> XADVAGTSNRDFRGREQRLFNSEQYNYNNSLNGEVSVWVYAYYSDGSVLVINKNSQYKVGISETFKALKEYREGQHNDSYDEYEVNQSIYYPNGGDARKFHSNAKPRAIQIIFSPSVNVRTIKMAKGNAVSVPDEYLQRSHPWEATGIKYRKIKRDGEIVGYSHYFELPHEYNSISLAVSGVHKNPSSYN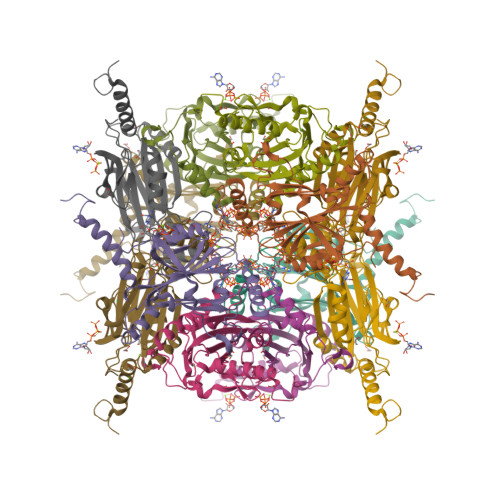VGGHNVMDVFQSCDLALRFCNRYWAELELVNHYISPNAYPYLDINNHSYGVALSNRQ>ASSAKFFVGGNWKSNGSVANVAKLVDELNAGTIPRGVDVVVAPPFIYIDYVMQHLDRDKYQLSAQNA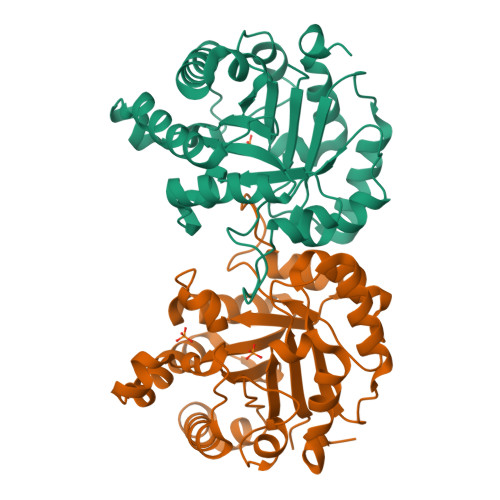WIGGNGAFTGEVSAEQLTDFGVPWVILGHSERRSLFGESNEVVAKKTSHALAAGLGVIACIGETLEQRNSGSVFKVLDAQMDALVDEVKDWTKVVLAYEPVWAIGTGVVASPEQAQEVHAYLRQYCAKKLGAAVADKLRIIYGGSVSDTNCKDLSKQEDIDGFLVGGASLKGAAFVTICNAAGPKAKP[2x]> EITRTTLQSDQEEIDYDDTISVEMKKEDFDIYDEDENQSPRSFQKKTRHYFIAAVERLWDYGMSSSPHVLRNRAQSGSVPQFKKVVFQEFTDGSFTQPLYRGELNEHLGLLGPYIRAEVEDNIMVTFRNQA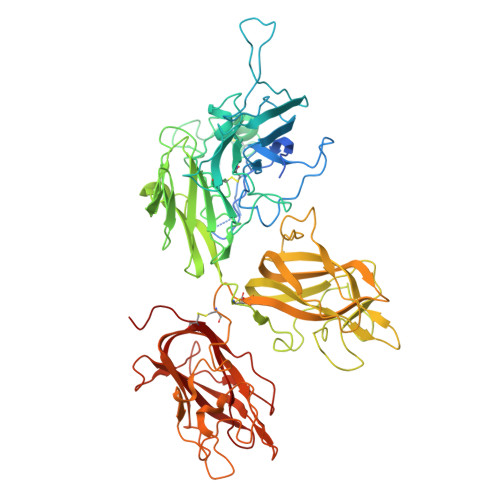SRPYSFYSSLISYEEDQRQGAEPRKNFVKPNETKTYFWKVQHHMAPTKDEFDCKAWAYFSDVDLEKDVHSGLIGPLLVCHTNTLNPAHGRQVTVQEFALFLTIFDETKSWYFTENMERNCRAPCNIQMEDPTFKENYRFHAINGYIMDTLPGLVMAQDQRIRWYLLSMGSNENIHSIHFSGHVFTVRKKEEYKMALYNLYPGVFETVEMLPSKAGIWRVECLIGEHLHAGMSTLFLVYSNKCQTPLGMASGHIRDFQITASGQYGQWAPKLARLHYSGSINAWSTKEPFSWIKVDLLAPMIIHGIKTQGARQKFSSLYISQFIIMYSLDGKKWQTYRGNSTGTLMVFFGNVDSSGIKHNIFNPPIIARYIRLHPTHYSIRSTLRMELMGCDLNSCSMPLGMESKAISDAQITASSYFTNMFATWSPSKARLHLQGRSNAWRPQVNNPKEWLQVDFQKTMKVTGVTTQGVKSLLTSMYVKEFLISSSQDGHQWTLFFQNGKVKVFQGNQDSFTPVVNSLDPPLLTRYLRIHPQSWVHQIALRMEVLGCEAQDLY> GSMTGPGALSGKVALVTGGSRGLGRAMALRLARDGAAVAIVYVSDDSSAKETQGEIERLGGTARSYRCDVSDAEQVTRCVKAVTADLGPVDILVNNAGIIRDGLAASIKDEDYDAVMNTNLKGAFLFIKACYFGFIRKRSGSIINISSVSGVFGSAGQANYASAKAGLIGLTKSIAKELAERNVRCNAVAPGLIATDMTQDLVDDSKRLDPVPMRRFGRPDEVAGLVAFLAGDESSYITGQVVCVDGGMAM

However, a recent study has shown that, in the biosynthesis of a symmetric polyketide dimer SIA7248, a trans-acting KR SiaM iteratively reduces the β-ketoacyl intermediates attached to different modules of the PKS. Here, we report the crystal structure of SiaM. The overall structure of SiaM resembles the consensus structure of KRs involved in the fatty acid biosynthesis as well as polyketide biosynthesis. It harbors a Rossmann fold which is responsible for the binding of NADPH molecules.

Although there is one SiaM molecule in each asymmetric unit, it forms a tetramer through symmetry operations. Superposition of SiaM, EryKR1, TylKR1 structures indicates that a variant form of LDD motif (IRD) can be found at the same location in SiaM. Noticeably, the second position of the LDD motif is occupied by a basic arginine residue, which has not been reported before. Instead of pointing towards the active site, the Arg99 is positioned towards solvent. Although SiaM crystallized without NADPH, the superposition of SiaM and other KR/NADPH complex structures indicates that NADPH binding cavity is present at the same location in the SiaM structure. Close to the NADPH binding site are the catalytic residues (Ser146, Tyr159, Lys163) that are conserved among KRs from various sources. In addition, a water molecule is found in the vicinity of conserved Lys163, which was proposed to be involved in the proton relay. As a result, the Tyr111 is located in the vicinity of the Phe123, which form aromatic stacking between them. Similarly, in the other interface of the tetramer, the aromatic stacking is found between Phe227 residues from neighboring protomers. In addition, Tyr235 inserts into the binding pocket in the opposite protomer and forms hydrogen bonds with the backbone carbonyl groups.>MSPILGYWKIKGLVQPTRLLLEYLEEKYEEHLYERDEGDKWRNKKFELGKHGHGHGKHKLEFPNLPYYIDGDVKLTQSMAIIRYIADKHNMLGGCPKERAEISMLEGAVLDIRYGVSRIAYSKDFETLKVDFLSKLPEMLKMFEDRLCHKTYLNGDHVTHPDFMLYDALDVVLYMDPMCLDAFPKLVCFKKRIEAIPQIDKYLKSSKYIAWPLQGWQATFGGGDHPPK[2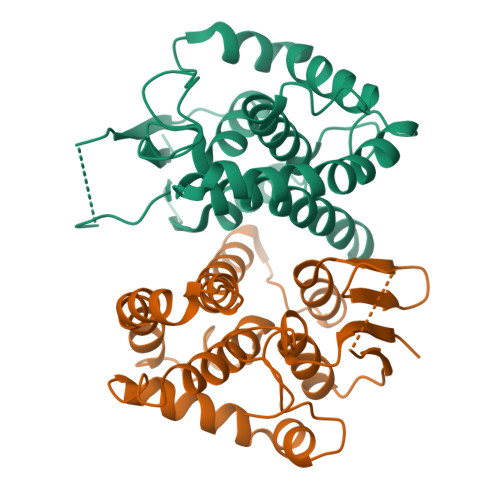x]>ALVFFAEDAGAIIGL[2x]

Amyloid-β (Aβ) forms heterogeneous oligomers, which are implicated in the pathogenesis of Alzheimer’s disease (AD). Peptides Aβm17–36 and Aβm17–35 mimic two different β-hairpins that Aβ can form, the Aβ17–36 and Aβ17–35 β-hairpins, respectively. These hairpins are similar in composition but differ in hairpin alignment, altering the facial arrangements of the side chains of the residues that they contain. Aβm17–36 and Aβm17–35 are cyclic hexadecapeptides consisting of two heptapeptide β-strands (Aβ17–23 and Aβ30–36 or Aβ29–35) connected by two δ-linked ornithine turn units that promote a β-hairpin-like conformation.

Aβm17–35 is designed to display the side chains of Met35, Gly33, Ile31, and Gly29 on the LFAD face and the side chains of Leu34, N-methyl-Ile32, and Ala30 on the VFE face. The X-ray crystallographic structure of Aβm17–35 contains two molecules of Aβm17–35 in the asymmetric unit. Both molecules fold to form twisted β-hairpins, and variation between the two monomers is minimal, consisting mainly of Met35 rotamers. The tetramers formed by Aβm17–35 consist of four β-hairpins arranged around a central axis to form a β-barrel. The tetramer can be viewed as a dimer of dimers in which two monomers assemble to form an antiparallel dimer, and two antiparallel dimers further assemble to form the tetramer. The hydrophobic side chains of the LFAD face comprise the core of the tetramer. The side chains of Phe19 and Met35 lie at the center of the hydrophobic core and are buttressed by the side chains of Leu17, Ala21, and Ile31. The absence of a side chain at Gly33 facilitates the tight packing of these hydrophobic side chains in a fashion similar to that previously reported for a cylindrin comprising three β-hairpins from αB crystallin. The charged residues Glu22 and Asp23 sit on the solvent-exposed ends of the Aβm17–35 cylindrin away from the hydrophobic core. Intermolecular hydrogen bonds between the monomer subunits further stabilize the tetramer.> MALTTTGTEQHDLFSGTFWQNPHPAYAALRAEDPVRKLALPDGPVWLLTRYADVREAFVDPRLSKDWRHTLPEDQRADMPATPTPMMILMDPPDHTRLRKLVGRSFTVRRMNELEPRITEIADGLLAGLPTDGPVDLMREYAFQIPVQVICELLGVPAEDRDDFSAWSSVLVDDSPADDKNAAMGKLHGYLSDLLERKRTEPDDALLSSLLAVSDEDGDRLSQEELVAMAMLLLIAGHETTVNLIGNGVLALLTHPDQRKLLAEDPSLISSAVEEFLRFDSPVSQAPIRFTAEDVTYSGVTIP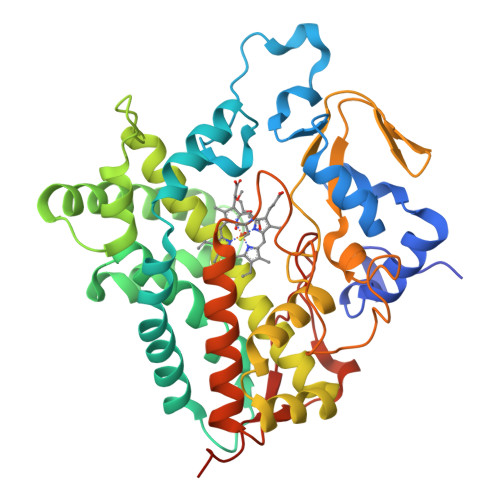AGEMVMLGLAAANRDADWMPEPDRLDITRDASGGVFFGHGIHFCLGAQLARLEGRVAIGRLFADRPELALAVGLDELVYRESTLVRGLSRMPVTMGPRSALEHHHHHH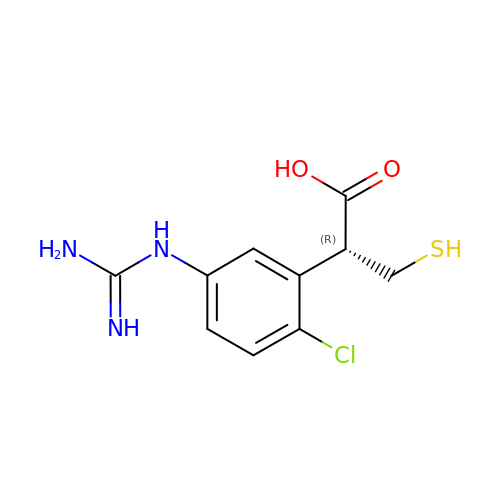2-(5-{[AMINO(IMINO)METHYL]AMINO}-2-CHLOROPHENYL)-3-SULFANYLPROPANOIC ACID | C10 H12 Cl N3 O2 S | DDXTYELBFUMBFH-SSDOTTSWSA-N>MHHHHHHMKDVIELTDDSFDKNVLDSEDVWMVEFY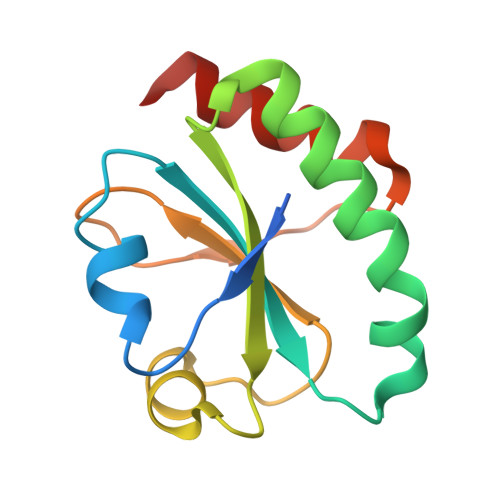APWCGHCKNLEPEWAAAASEVKEQTKGKVKLAAVDATVNQVLASRYGIRGFPTIKIFQKGESPVDYDGGRTRSDIVSRALDLFSDNAP[2x]>[28x]MADSDINIKTGTTDIGSNTTVKTGDLVTYDKENGMHKKVFYSFIDDKNHNKKLLVIRTKGTIAGQYRVYSEEGANKSGLAWPSAFKVQLQLPDNEVAQISDYYPRNSIDTKEYMSTLTYGFNGNVTGDDTGKIGGLIGANVSIGHTLKYVQPDFKTILESPTDKKVGWKVIFNNMVNQNWGPYDRDSWNPVYGNQLFMKTRNG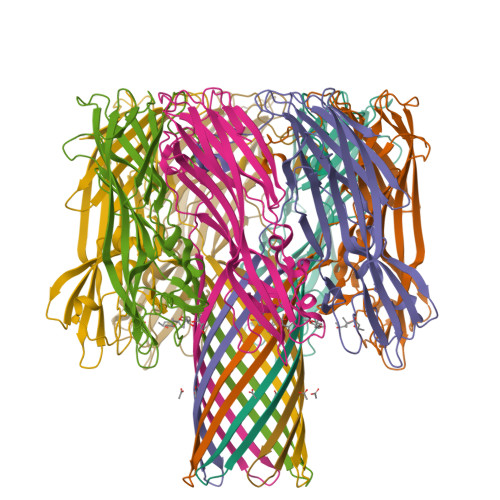SMKAAENFLDPNKASSLLSSGFSPDFATVITMDRKASKQQTNIDVIYERVRDDYQLHWTSTNWKGTNTKDKWTDRSSERYKIDWEKEEMTNLEHHHHHH>AEHIVEMRNKDDAGNTMVFQPGFVKVEAGDTVKFVPTDKSHNAESVREVWPEGVAPVKGGFSKEV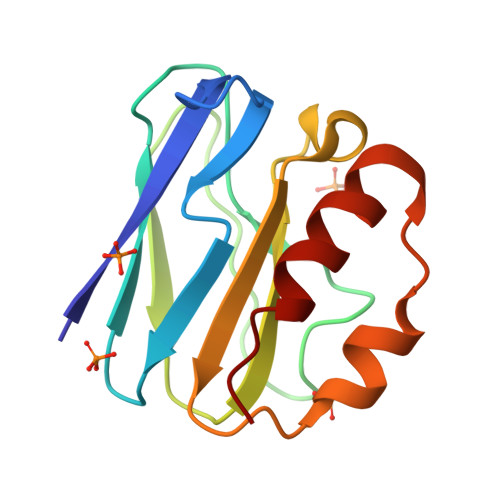VFNAEKEGLYVLKCAPHYGMGMVVLVQVGKPVNLDQIKEYKATGLAKKRLDGEIAKVVQ[3x]> MRRCTVARYYWSRYRIPSQMPKFDGPAPVAAPQNMNSTKTNEFIDPIDDKFPVTIRGNLVRPDVPEDQYVDSWYVCTSMTHHLGDFRPWSASAPANAYRFRPYNEFDSKGREYVEHLRKYSRYTPQASRGKGANGFPFREAFLTKMNTAETAAVNPTRETVMTRAVAERLHHARVLSPLEVQRDVGRLEEPLPCAGKIPAERSTFPFRWNTEDWYEYEVAKARNKRFVFENTNDNGVCASEVTYRIVLEGFWDHHVMKLADDVVMFLKDVGRQVVDEKLKSVRASLESLSSGGAVDPELVAAFNASLKGPFGGADRYDADEVAHFLRSELERLEEQCVGLINRANVPIPGTSNIYDANVSWPHVEKMEPWTRMAEFWTSSSDTSFTELEMSTAHYEFRKYFRVVVVKMPFQSTEFEQRMYGIRHWLHRQTSCEFHTTYRRNVVHDSAVFPTEHDPETKPSHEHHRLFSFALDWQSAPVDYLSVELAREGDSWSSLAKRLGCSESELKAANGAMEEVVAGVAVSVPGSATRRLTSFSTTPSVLPLQQGDGKPAITSWRRAAEVLGCSVEELQQANGAAALTYMAAAESGDGAFDPAIKELVVPHTATAASPESSFAAFEPVFEGDTWTSIAARLGCSEADLRACNDVDGSVADVSSCASVSVPASATRPRRIIHPQLRPQAATDALLARTLGEQAVSAMGDIPSLPANAHKFPHEYHTPTSRFPTTPQQSPASDNWIAYTAKYLDKQLALQDEPATVYNVNKLWPMQQVPGKVDQTPFEEDQT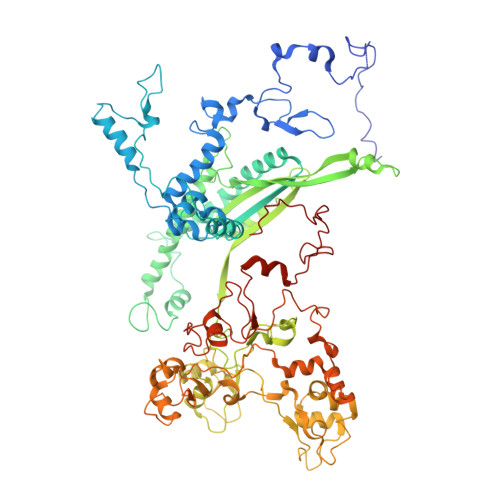WLMHPIPVHQMQQHHPEKDLQDLPFVNHEQFPRSLEWTAP>GIGTGFPFDPHYVEVLGERMHYVDVGPRDGTPVLFLHGNPTSSYVWRNIIPHVAPTHRCIAPDLIGMGKSDKPDLGYFFDDHVRFMDAFIEALGLEEVVLVIHDWGSALGFHWAKRNPERVKGIAFMEFIRPIPTWDEWPEFARETFQAFRTTDVGRKLIIDHNVFIEGTLRMGVVRPLTEVEMDHYREPFLNPVDREPLWRFPNELPIAGEPANIVALVEEYMDWLHQSPVPKLLFWGTPGVLIPPAEAARLAKSLPNCKAVD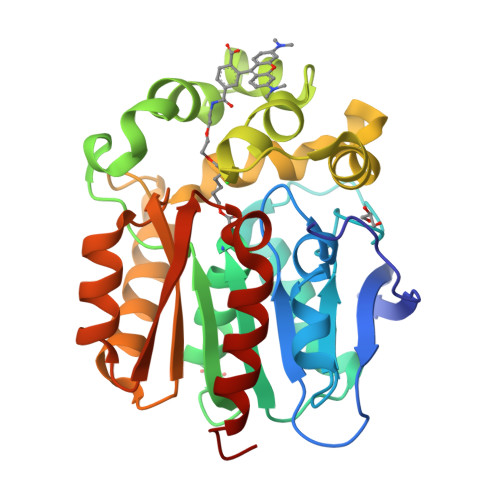IGPGLNLLQEDNPDLIGSEIARWLSTLEI[2x]(2~{S})-2-[2-(4-chlorophenyl)sulfanylethanoylamino]-3-methyl-butanoic 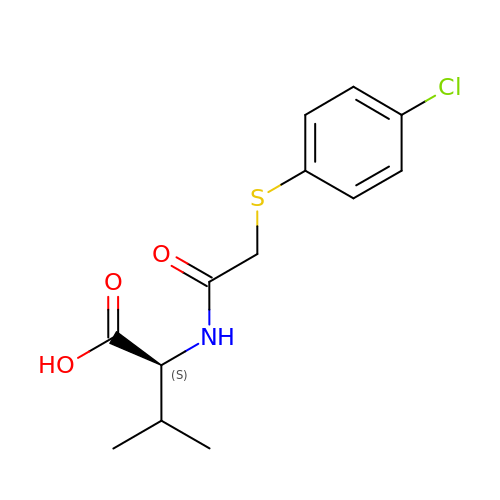acid | C13 H16 Cl N O3 S | IKYARSKDJJAPDW-LBPRGKRZSA-N>[8x]TENKRKSMEKLSVDGVISALAFDQRGALKRMMAQHQTKEPTVEQIEELKSLVSEELTPFASSILLDPEYGLPASRVRSEEAGLLLAYEKTGYDATTTSRLPDCLDVWSAKRIKEAGAEAVK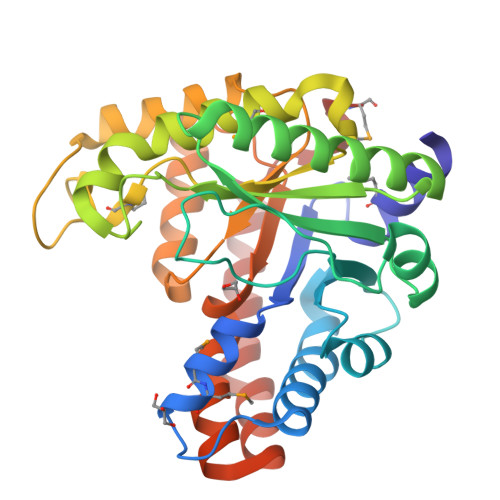FLLYYDIDGDQDVNEQKKAYIERIGSECRAEDIPFYLEILTYDEKIADNASPEFAKVKAHKVNEAMKVFSKERFGVDVLKVEVPVNMKFVEGFADGEVLFTKEEAAQAFRDQEASTDLPYIYLSAGVSAKLFQDTLVFAAESGAKFNGVLCGRATWAGSVKVYIEEGPQAAREWLRTEGFKNIDELNKVLDKTASPWTEKM> MPKSMNVRVTTMDAELEFAIQQTTTGKQLFDQVVKTIGLREVWFFGLQYTDSKGDLTWIKLYKKVMQQDVKKENPLQFKFRAKFYPEDVADELIQEITLKLFYLQVKNAILSDEIYCPPETSVLLASYAVQARHGDHNPAVHGPGFLANDRLLPQRVTDQHKMSREEWEQSITNWWQEHRGMLREDAMMEYLKIAQDLEMYGVNYFEIRNKKNTELWLGVDALGLNIYEKDDKLTPKIGFPWSEIRNISFNDRKFIIKPIDKKAPDFVFFAPRVRVNKRILALCMGNHELYMRRRKPDTIDVQQMKAQAREEKLAKQAQREKLQLEIAARERAEKKQQEYQDRLRQMQEEMERSQANLLEAQDMILRLEEQLRQLQAAKEELEQRQNELQAMMQRLEETKNMEAAERQKLEDEIRAKQEEVSRIQQEVELKDSETRRLQEEVEDARRKQDEAAAALLAATTPQHHHVAERADTDPDHDNASDAGSESGGGDLARGPDDLVDPVADRRTLAERNERLHNQLKA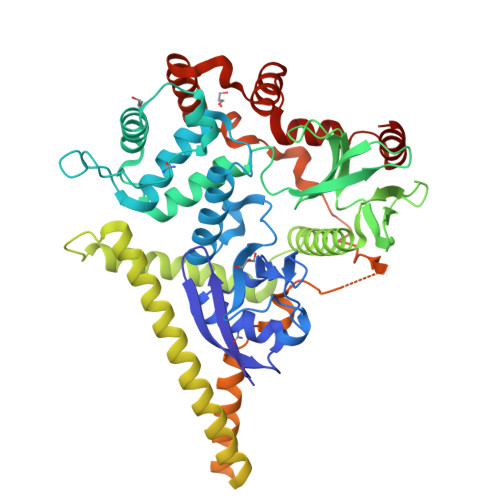LKQDLARSCDETKETAMDKIHRENVRQGRDKYKTLREIRKGNTKRRVDQFENM>[2x]SMLWVGVVSIFPEMFRAISDYGITSRAVKQGLLTLTCWNPRVYTEDRHQTVDDRPFGGGPGM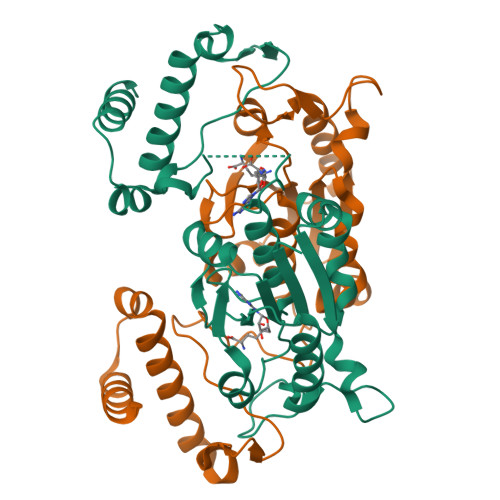VMKIKPLEGALADARQAAGGRKAKVIYLSPQGRQLTQAGVRELAEEEALILIAGRYEGIDERFIEEHVDEEWSIGDYVLSGGELPAMVLVDAVTRLLPGALGHADSAEEDSFTDGLLDCPHYTRPEVYADKRVPEVLLSGNHEHIRRWRLQQALGRTWERRADLLDSRSLSGEEQKLLAEYIRQRD>[2x]QKTKQFSVPNLPLNVMSNSRVPSLLNAMVVSPDQAQVVQFQNGRCTLDGQMLGTTTVSASCVARFRGKTFQAPDNRLGINLAEISGEPYHAFESPAPLGFPDFGDGDWHVTATKVTPSQLEANDPVVVGNVQPYNPQFAPHLGTLVVENPTPDQVATGTDLLFNITWLSNRANNRFNPWVIPNYGSTLTEAAQLAPSIFPPGFGETIVYFNSTFPAVGATTHAAIPCLLPQEFVAHFVNEQAPIRGEAALLHYIDPDTHRNLGEFKIYPEGFVTCVPNVGGTGPQSLPTNGVFVFVSWVSRYYQLKPVGTAG

Noroviruses have been identified as major causative agents of acute nonbacterial gastroenteritis in humans. Histo‐blood group antigens (HBGAs) are thought to play a major role among the host cellular factors influencing norovirus infection. Genogroup I, genotype 9 (GI.9) is the most recently identified genotype within genogroup I, whose representative strain is the Vancouver 730 norovirus. We determined the crystal structures of the protruding domain of the GI.9 capsid protein in the presence or absence of Lewis antigens.

However, the molecular interactions between host antigens and the GI.9 capsid protein have not been investigated in detail.>[5x]MPTSNPAKPLDGFRVLDFTQNVAGPLAGQVLVDLGAEVIKVEAPGGEAARQITSVLPGRPPLATYFLPNNRGKKSVTVDLTTEQAKQQMLRLADTADVVL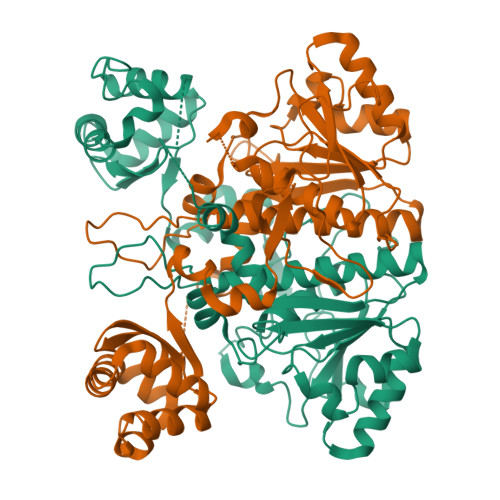EAFRPGTMEKLGLGPDDLRSRNPNLIYARLTAYGGNGPHGSRPGIDLVVAAEAGMTTGMPTPEGKPQIIPFQLVDNASGHVLAQAVLAALLHRERNGVADVVQVAMYDVAVGLQANQLMMHLNRAASDQPKPEPAPKAKRRKGVGFATQPSDAFRTADGYIVISAYVPKHWQKLCYLIGRPDLVEDQRFAEQRSRSINYAELTAELELALASKTATEWVQLLQANGLMACLAHTWKQVVDTPLFAENDLTLEVGRGADTITVIRTPARYASFRAVVTDPPPTAGEHNAVFLARP>[3x]GAMEMLPNQTIYINNLNEKIKKEELKKSLYAIFSQFGQILDIVALKTLKMRG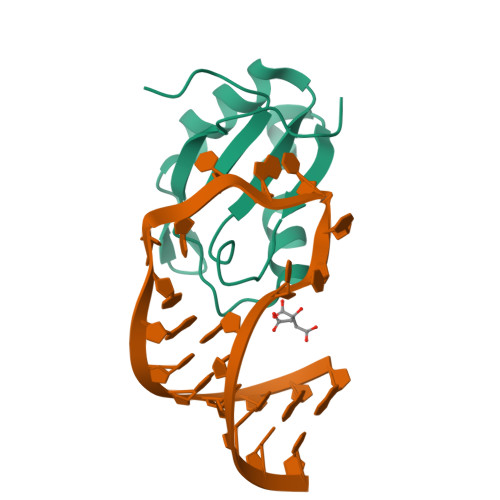QAFVIFKEIGSASNALRTMQGFPFYDKPMQIAYSKSDSDIVAKIKG> SNAMKMSELEKMLKGEHFDGASAEIEALRSQAGRLKLEINQSLDEAERYALQREL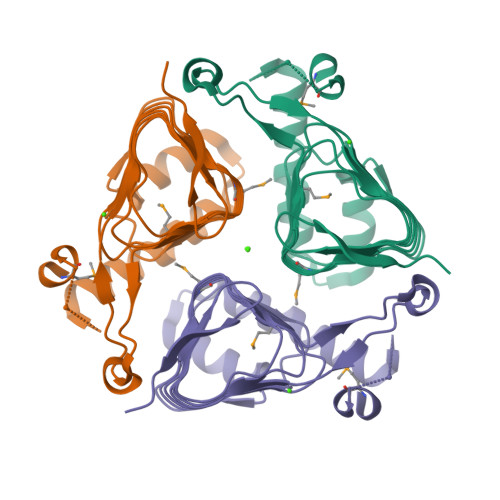FGHLGHKSCVQPPFHCEFGKTIRIGDHTFINMNVVMLDGAPITIGDHVLIGPSTQFYTASHSLDYRRRQAWETICKPIVIEDDVWIGGNVVINQGVTIGARSVVAANSVVNQDVPPDTLVGGTPARILRSLKDPAESMAE> MKQALRVAFGFLILWASVLHAEVRIVIDSGVDSGRPIGVVPFQWAGPGAAPEDIGGIVAADLRNSGKFNPLDRARLPQQPGSAQEVQPAAWSALGIDAVVVGQVTPNPDGSYNVAYQLVDTGGAPGTVLAQNSYKVNKQWLRYAGHTASDEVFEKLTGIKGAFRTRIAYVVQTNGGQFPYELRVSDYDGYNQFVVHRSPQPLMSPAWSPDGSKLAYVTFESGRSALVIQTLANGAVRQVASFPRHNGAPAFSPDGSKLAFALSKTGSLNLYVMDLASGQIRQVTDGRSNNTEPTWFPDSQNLAFTSDQAGRPQVYKVNINGGAPQRITWEGSQNQDADVSSDGKFMVMVSSNGGQQHIAKQDLATGGVQVLSSTFLDETPSLAPNGTMVIYSSSQGMGSVLNLVSTDGRFKARLPATDGQVKFPAWSPYLLEHHHHHH;> MPGFNYGGKGDGTGWSSERGSGPEPGGGSHGNSGGHDRGDSSNVGNESVTVMKPGDSYNTPWGKVIINAAGQPTMNGTVMTADNSSMVPYGRGFTRVLNSLVNNPVSLEHHHHHH

Colicins are plasmid-encoded, protein antibiotics that consist of three domains; an N-terminal translocation (T) domain, a central receptor-binding (R) domain and a C-terminal cytotoxic domain. To facilitate import of their cytotoxic domains to their cellular site of action, group A colicins, such as the E colicins and colicin A (ColA), use the tol-dependent translocation system that consists of the TolQ, TolR, TolA, TolB and Pal proteins, and constitutes a transmembrane protein translocation portal or translocon. TolB is a periplasmic protein, whose crystal structure was independently determined by two groups, and is associated with the outer membrane via an interaction of its C-terminal β-propeller domain with the peptidoglycan-associated lipoprotein (Pal), and with TolA via its N-terminal domain. ColA interacts with TolB through a TolB box (DGTGW), that has been localized to residues 11–15 in the T domain of ColA and shares high sequence homology with part of the TolB box of other group A colicins such as ColE9 (DGSGW).

In this paper we have used site-directed mutagenesis data together with the elucidation of the cocrystal structure of a TolB box containing peptide consisting of the N-terminal 107 residues of ColA (TA1–107) bound to TolB to show that the TolB box of ColA consists of a 12-residue domain that binds to the β-propeller canyon of TolB. The structure was refined to 2.6 Å resolution; and the model has excellent geometry with no Ramachandran outliers. Even though 107 amino acids of the translocation domain of ColA were included in the crystallization, only residues 9–20 could be resolved in the electron density maps. Our final colicin model fitted the density very well, with clean difference maps. TolB, as previously described, is composed of an α/β domain at the N terminus and a six-bladed β-propeller domain at the C terminus with a tunnel through the centre of the β-propeller. Refinement of two small, independent peaks of positive density using water, monovalent and divalent cations suggested that one Ca2+ ion is present in the central channel of the β-propeller and a Na+ ion is present at the interface between the N-terminal α/β domain and β-propeller domain. Our structure of the complex of TolB and TA1–107 has revealed that the TolB box in ColA is a 12-residue peptide with the sequence of 9-KGDGTGWSSERG-20. The TolB box core of ColA forms an O ring shape, due to the hydrogen bond between the D11 and the E18 residues, and sits at the bottom of the tunnel in TolB with six hydrogen bonds stabilizing the interaction with TolB. The first set of interactions are predominantly hydrophobic in nature, with only one hydrogen bond between W15 of ColA and D307 of TolB.> GPESAPRIMRLVAECSRSGARAGELRLPHGTVATPVFMPVGTQATMKGITTEQLDSLGCRICLGNTYHLGLRPGPELIRKAQGLHGFMNWPHNLLTDSGGFQMVSLFSLSEVTEEGVHFRSPYDGEETLLSPERSV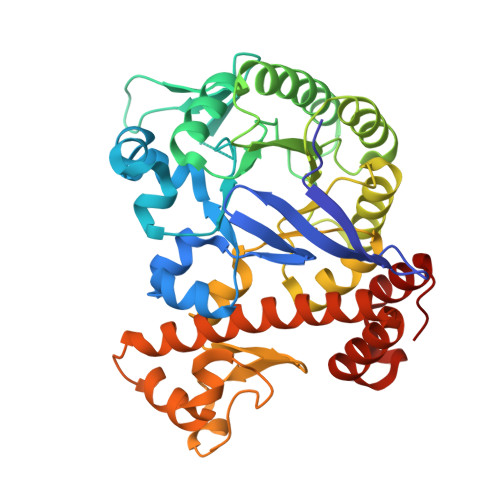EIQNALGSDIIMQLDHVVSSTVTGPLVEEAMHRSVRWLDRCIAAHKHPDKQNLFAIIQGGLNADLRTTCLKEMTKRDVPGFAIGGLSGGESKAQFWKMVALSTSMLPKDKPRYLMGVGYATDLVVCVALGCDMFDCVYPTRTARFGSALVPTGNLQLKKKQYAKDFSPINPECPCPTCQTHSRAFLHALLHSDNTTALHHLTVHNIAYQLQLLSAVRSSILEQRFPDFVRNFMRTMYGDHSLCPAWAVEALASVGIMLT>[3x]DYDQ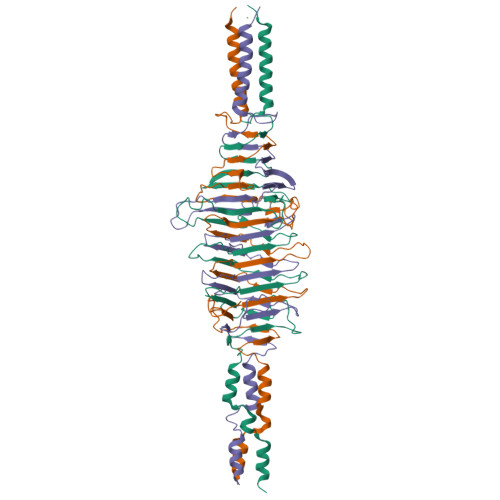LQNKPDLGAFAQKEETNSKITKLESSKADKSAVYSKAESKIELDKKLSLTGGIVTGQLQFKPNKSGIKPSSSVGGAINIDMSKSEGAAMVMYTNKDTTDGPLMILRSDKDTFDQSAQFVDYSGKTNAVNIVMRQPSAPNFSSALNITSANEGGSAMQIRGVEKALGTLKITHENPNVEAKYDENAAALSIDIVKKQKGGKGTAAQGIYINSTSGTAGKMLRIRNKNEDKFYVGPDGGFHSGANSTVAGNLTVKDPTSGKHAATKDYVDEKIAELKKLILKKLEHHHHHH> MDNIIMTAYISIFVQIITAIISVYGLFIPLNFKDIILREILILELIVQIIEFIFYIWLIITLQSINEDITYVRYFDWVLTTPVMLLTTVYFFEYMNSDDGIRKKEINDRDYVYLFYICLSNFFMLLIGYLGETKQINKMLTLFGGSFFLFLTFYLLYVKYTKENWMNYIVFYFMFLVWFLYGFAFMFPFSIKNQMYNILDIVSKNIYSIFI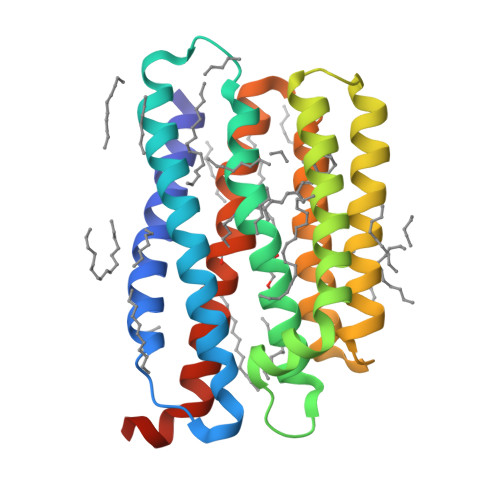FIVILNQSYKLLLEHHHHHH R.PabI is a type II restriction enzyme from the hyperthermophilic archaea Pyrococcus abyssi and belongs to the HALFPIPE superfamily. R.PabI recognizes the 5′-GTAC-3′ sequence and cleaves the N-glycosidic bond of the adenine in the recognition sequence. The structural analysis of R.PabI showed that R.PabI forms a dimer and possesses a characteristic highly curved β sheet, called the half-pipe structure, at the protomer-protomer interface. The N-glycosidic bond of the flipped adenine is cleaved by R.PabI by hydrolysis, similarly to DNA glycosylases.

In this study, we determined the crystal structure of R.PabI in complex with 20 base pairs of dsDNA, not containing the R.PabI recognition sequence, to uncover how R.PabI interacts with nonspecific dsDNA. To determine the R.PabI-nonspecific dsDNA complex structure, we utilized the R32A E63A double mutant of R.PabI, which contains residues 8-226. In this study, we determined the structure of R.PabI in complex with 20 bp of dsDNA at 1.9 Å resolution. The asymmetric unit of the crystal contains one R.PabI dimer (protomers A and B), one single-stranded DNA (ssDNA, chain C), and 162 water molecules. The R.PabI-ssDNA complex observed in the asymmetric unit forms a tetrameric R.PabI structure with a symmetrically related complex generated by the crystallographic two-fold axis (R.PabI protomers A’ and B’ and ssDNA strand C’). In the tetrameric structure, the 20 bp dsDNA is sandwiched by the half-pipe regions of two R.PabI dimers. Although the contact surface area between the two protomers is small (the contact surface areas between the A-A’ and B-B’ interfaces are 201.1 Å2 and 102.8 Å2, respectively), the two R.PabI dimers are connected by four salt bridges between the protomers. The interface area between the R.PabI dimer and the dsDNA in the nonspecific complex is 1156 Å2, which is approximately half of the interface area in the specific complex (2166 Å2). In the R.PabI-nonspecific dsDNA complex structure, the dsDNA is recognized by 24 hydrogen bonds between the DNA and each R.PabI dimer. The structure of dsDNA between the two R.PabI dimers is slightly bent by ~20o at its middle region due to these R.PabI-nonspecific dsDNA interactions.

>MEASVSFENGKIVVRLPITRPTSKIAVKKIENGVGIPVSTRKKSFPSDENLRDYYIAWQISYARDGKYDYELSRMVRLAHEHGILTYNDIYELLKFADDVKSYLEDKGIRRESTNEELYGFNIYEDVYPVAKKELPSGEFIGIVLKHKQRAVGYQSMVYVCIPLTNVEPSLAGRVARRNEVVKYEVPVDLMKELLKAFIIASETHKNDIVKFLRSIIGTS[2x]>SN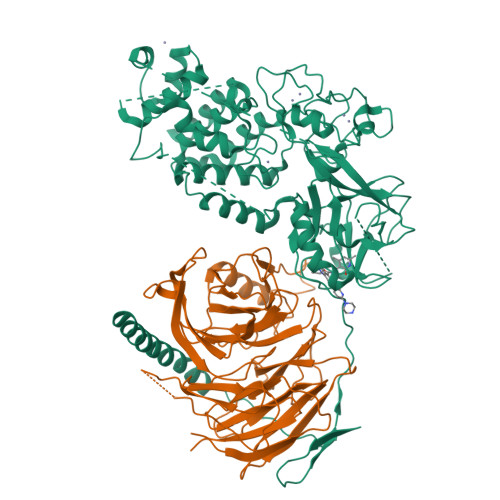AHHHHHHGQTGKKSEKGPVCWRKRVKSEYMRLRQLKRFRRADEVKSMFSSNRQKILERTEILNQEWKQRRIQPVHILTSVSSLRGTRECSVTSDLDFPTQVIPLKTLNAVASVPIMYSWSPLQQNFMVEDETVLHNIPYMGDEVLDQDGTFIEELIKNYDGKVHGDRECGFINDEIFVELVNALGQYNREEKQKDLEDHRDDKESRPPRKFPSDKIFEAISSMFPDKGTAEELKEKYKELTEQQLPGALPPECTPNIDGPNAKSVQREQSLHSFHTLFCRRCFKYDCFLHPFHATPNTYKRKNTETALDNKPCGPQCYQHLEGAKEFAAALTAERIKTPPKRPGGRRRGRLPNNSSRPSTPTINVLESKDTDSDREAGKPNIEPPENVEWSGAEASMFRVLIGTYYDNFCAIARLIGTKTCRQVYEFRVKESSIIAPAPAEDVDTPPRKKKRKHRLWAAHCRKIQLKKDGSSNHVYNYQPCDHPRQPCDSSCPCVIAQNFCEKFCQCSSECQNRFPGCRCKAQCNTKQCPCYLAVRECDPDLCLTCGAADHRDSKNVSCKNCSIQRGSKKHLLLAPSDVAGWGIFIKDPVQKNEFISEYCGEIISQDEADRRGKVYDKYMCSFLFNLNNDFVVDATRKGNKIRFANHSVNPNCYAKVMMVNGDHRIGIFAKRAIQTGEELFFDYRYSQADALKYVGIEREMEIPFLESEDGEVEQQRTYSSGHNRLYFHSDTCLPLRPQEMEVDSEDEKDPEWLREKTITQIEEFSDVNEGEKEVMKLWNLHVMKHGFIADNQMNHACMLFVENYGQKIIKKNLCRNFMLHLVSMHDFNLISIMSIDKAVTKLREMQQKLEKGESAS[2x];>[2x]MSSEREVSTAPAGTDMPAAKKQKLSSDENSNPDLSGDENDDAVSIESGTNTERPDTPTNTPNAPGRKSWGKGKWKSKKCKYSFKCVNSLKEDHNQPLFGVQFNWHSKEGDPLVFATVGSNRVTLYECHSQGEIRLLQSYVDADADENFYTCAWTYDSNTSHPLLAVAGSRGIIRIINPITMQCIKHYVGHGNAINELKFHPRDPNLLLSVSKDHALRLWNIQTDTLVAIFGGVEGHRDEVLSADYDLLGEKIMSCGMDHSLKLWRINSKRMMNAIKESYDYNPNKTNRPFISQKIHFPDFSTRDIHRNYVDCVRWLGDLILSKSCENAIVCWKPGKMEDDIDKIKPSESNVTILGRFDYSQCDIWYMRFSMDFWQKMLALGNQVGKLYVWDLEVEDPHKAKCTTLTHHKCGAAIRQTSFSRDSSILIAVCDDASIWRWDRLR>MNVRVLVVEDERDLADLITEALKKEMFTVDVCYDGEEGMYMALNEPFDVVILDIMLPVHDGWEILKSMRESGVNTPVLMLTALSDVE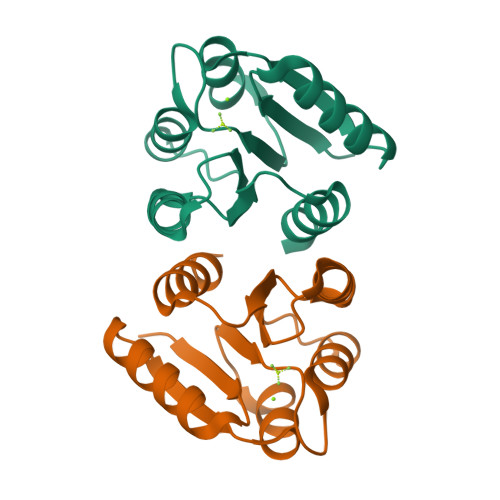YRVKGLNMGADDYLPKPFDLRELIARVRALIRRKS[2x]>MASSAQDGNNPLFSPYKMGKFNLSHRVVLAPMTRCRALNNIPQAALGEYYEQRATAGGFLITEGTMISPTSAGFPHVPGIFTKEQVREWKKIVDVVHAKGAVIFCQLWHVGRASHEVYQPAGAAPISSTEKPISNRWRILMPDGTHGIYPKPRAIGTYEISQVVEDYRRSALNAIEAGFDGIEIHGAHGFLIDQFLKDGINDRTDEYGGSLANRCKFITQVVQAVVSAIGADRVGVRVSPAIDHLDAMDSNPLSLGLAVV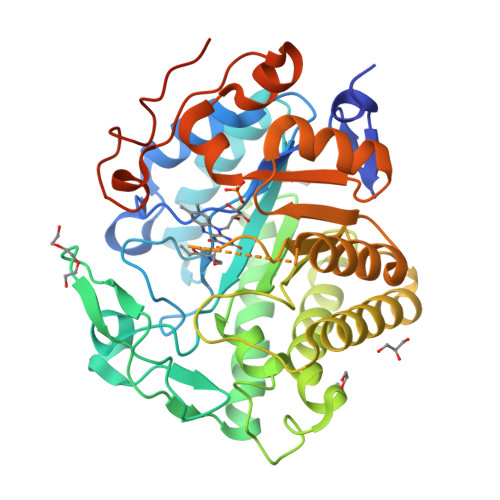ERLNKIQLHSGSKLAYLHVTQPRYVAYGQTEAGRLGSEEEEARLMRTLRNAYQGTFICSGGYTRELGIEAVAQGDADLVSYGRLFISNPDLVMRIKLNAPLNKYNRKTFYTQDPVVGYTDYPFLQGNGSNGPLSRLLEHHHHHH[2x]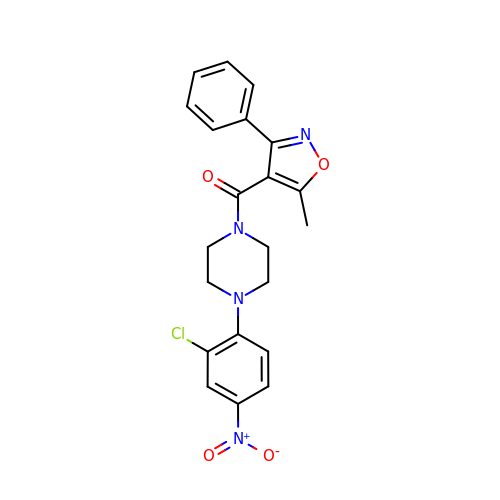[4-(2-chloro-4-nitrophenyl)piperazin-1-yl](5-methyl-3-phenyl-1,2-oxazol-4-yl)methanone | C21 H19 Cl N4 O4 | OWXBJAPOSQSWAO-UHFFFAOYSA-N> SE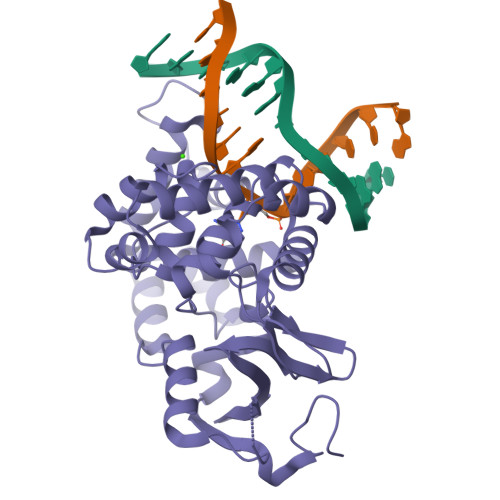FGHRTLASTPALWASIPCPRSELRLDLVLPSGQSFRWREQSPAHWSGVLADQVWTLTQTEEQLHCTVYRGDKSQASRPTPDELEAVRKYFQLDVTLAQLYHHWGSVDSHFQEVAQKFQGVRLLRQDPIECLFSFICSSCNNIARITGMVERLCQAFGPRLIQLDDVTYHGFPSLQALAGPEVEAHLRKLGLGYRARYVSASARAILEEQGGLAWLQQLRESSYEEAHKALCILPGVGTQVADCICLMALDKPQAVPVDVHMWHIAQRDYSWHPTTSQAKGPSPQTNKELGNFFRSLWGPYAGWAQAVLFSADLRQSR>[4x]MATSGFSKPLHYPPVRRDETVVDDYFGVKVADPYRWLEDPNSEETKEFVDNQEKLANSVLEECELIDKFKQKIIDFVNFPRCGVPFRRANKYFHFYNSGLQAQNVFQMQDDLDGKPEVLYDPNLREGGRSGLSLYSVSEDAKYFAFGIHSGLTEWVTIKILKTEDRSYLPDTLEWVKFSPAIWTHDNKGFFYCPYPPLKEGEDHMTRSAVNQEARYHFLGTDQSEDILLWRDLENPAHHLKCQITDDGKYFLLYILDGCDDANKVYCLDLTKLPNGLESFRGREDSAPFMKLIDSFDASYTAIANDGSVFTFQTNKDAPRKKLVRVDLNNPSVWTDLVPESKKDLLESAHAVNENQLILRYLSDVKHVLE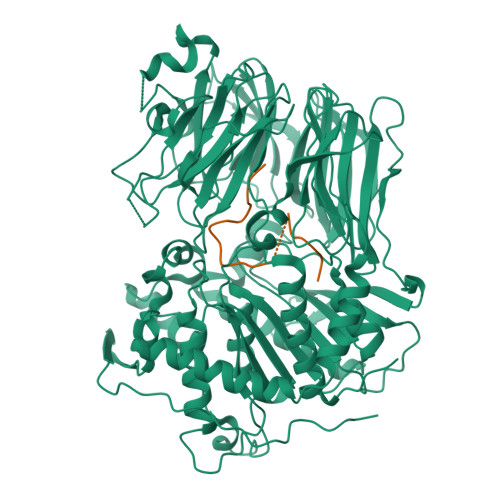IRDLESGALQHRLPIDIGSVDGITARRRDSVVFFKFTSILTPGIVYQCDLKNDPTQLKIFRESVVPDFDRSEFEVKQVFVPSKDGTKIPIFIAARKGISLDGSHPCEMHGYGGFGINMMPTFSASRIVFLKHLGGVFCLANIRGGGEYGEEWHKAGFRDKKQNVFDDFISAAEYLISSGYTKARRVAIEGGANGGLLVAACINQRPDLFGCAEANCGVMDMLRFHKFTLGYLWTGDYGCSDKEEEFKWLIKYSPIHNVRRPWEQPGNEETQYPATMILTADHDDRVVPLHSFKLLATMQHVLCTSLEDSPQKNPIIARIQRKAAHYGRATMTQIAEVADRYGFMAKALEAPWID;>MATSFQFDGLKPSFSASYSSKPIQTQVSNGMDNASAPV[4x]>[2x]HHHHHH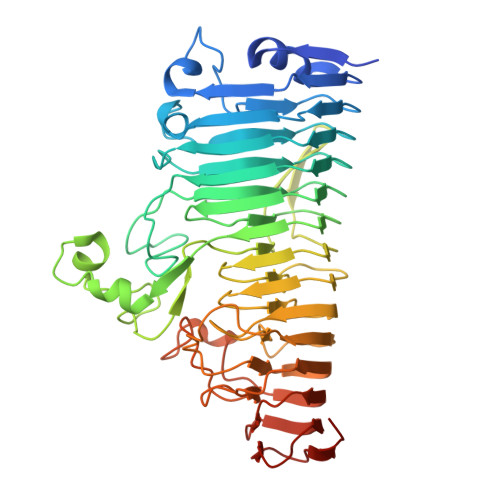SSGLVPRGSHMQTTTVYSLEDLLPYLKQDNVDVKLAPGTYNVNGFDVGEDRLFSTTPLFLFEGSNSTYDFTDVKLNINTVVLTKFGNNEVNEIQILGNNNVLKNLKLEDIGTTAPSNRAQSIVIDGRDNRIEGFHLTIRGSYPYGYGDAFGKGGGSVINHRKHSGVLIRGLRNHLKDCTIISRSYGHIVFMQAASYPTVEGCYIEGEMRSTDDMLAEEGTGSPADKVDFMTVWGYKLPAGYMMSLQEGGIRAFNAGTTYIDGVEIQRATDNPTVLNCTIKNARTGVTLAHANGTKYVEGCTVLGCENGYSIGSGTVVNCGADAIYGPVFKNTYGSDKGYNADITILPPSDAYYNGHDAVAYIGGSNHNLTFRSEITEIPSNLKIMVSGDLQGLRVLHGSNPSQNNFAGTNIVLRNLTNFPVDLHSDSSNITVTSCDTDNITDNGTNNSIEAIDCDSD>INAEKPNVRFKDMAGNEEAKEEVVEIVDFLKYPERYANLGAKIPKGVLLVGPPGTGKTLLAKAVAGEAHVPFFSMGGSSFIEMFVGLGASRVRDLFETAKKQAPSIIFIDEIDAIGKSRAAGGVVSGNDEREQTLNQLLAEMDGFGSENAPVIVLAATNRPEILDPALMRPGRFDRQVLVDKPDFNGRVEILKVHIKGVKLANDVNLQEVAKLTAGLAGADLANIINEAALLAGRNNQKEV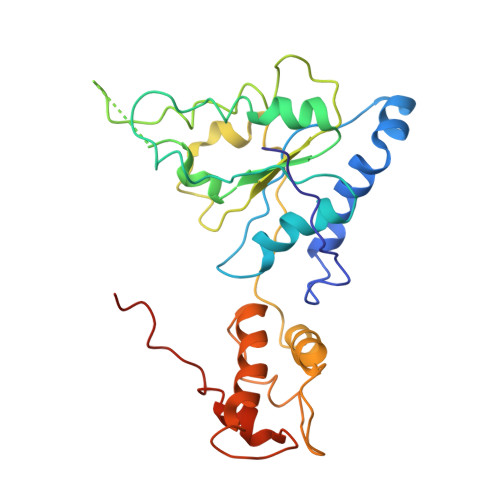RQQHLKEAVERGIAGLEKKLEHHHHHH[2x]>GMATPKKDVYTIASDNSFAPFEFQNDDKQFTGIDVDLLNAIAKNQGFKLKWNFIGFQAAVDSVQSGHADGMMSGMSITDARKQVFDYGSPYYSSNLTIATSSTDDSIKSWKDLKGKTLGAKNGTASFDYLNAHAKEYGYTVKTFTDATTMYSS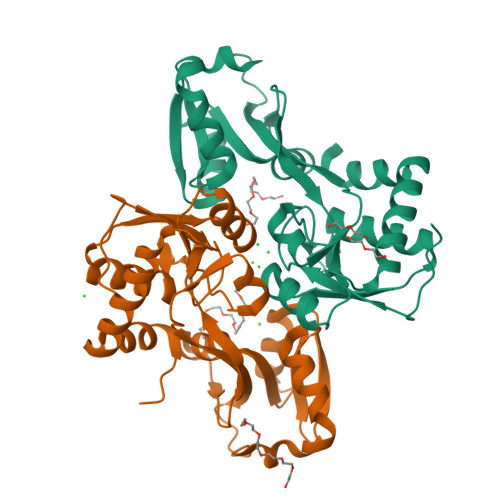LNNGSINALMDDEPVIKYAIKQGQKFATPIKPIPDGQYGFAVKKGSNPELIEMFNNGLANLRANGEYDKIIDKYLESDA[2x]Mutations in the human PURA gene cause the neurodevelopmental PURA syndrome. Based on the crystal structures of PURA from Drosophila melanogaster (dmPURA), three conserved sequence regions termed PUR repeats I, II, and III were identified to fold into globular domains. Whereas PUR repeat I and II assemble into an N-terminal PUR domain via intramolecular interactions, two C-terminal PUR repeats III from different molecules interact with each other and thus mediate dimerization of PURA. All these PUR domains belong to the class of the PC4-like protein family, which mainly bind single-stranded nucleic acids and can unwind double-stranded DNA and RNA.

Since Drosophila and human PURA have a rather moderate sequence identity of 46%, we decided to establish a better experimental basis for predicting the structural effects of patient-derived genetic variations and determined the crystal structure of the fragment P215-K280 (i.e. hsPURA III) at 1.7 Å resolution. The structure of the C-terminal PUR-domain possesses the typical four antiparallel β-strands and one α-helix. Like in the previously published dmPURA III structure, the C-terminal PUR domain of hsPURA is built from two PUR repeats III of independent protein chains that interact with each other to form an intermolecular homodimer. The hsPURA III dimer shows high structural similarity to dmPURA III with root mean square deviation (r.m.s.d.) of 1.26 Å for 125 superimposed Cα atoms and 50% of sequence identity. Analysis of the crystal structure of the hsPURA III homodimer revealed electrostatic surface potentials favorable for interactions with nucleic acids. When performing gel electrophoresis mobility shift assays (EMSAs) we indeed observed RNA binding. We indeed observed strand separation in presence of the hsPURA III fragment. F233 is part of the β-sheet and interacts with the α-helix of the other PUR repeat III within the PUR domain, contributing to dimerization. Since in the PURA F233del variant, one residue is deleted, the orientation of all subsequent amino acids in the β-strand adopt the opposite orientation, likely resulting in a fold disruption of the β-sheet and possibly in impaired dimerization. In the case of the R245P variant, the exchange into proline also likely impairs β-strand folding by introducing a kink, which could also impact dimerization.

>[2x]GPMAELPEGTSLTVDNKRFFFDVGSNKYGVFMRVSEVKPTYRNSITVPYKVWAKFGHTFCKYSEEMKK>[6x]M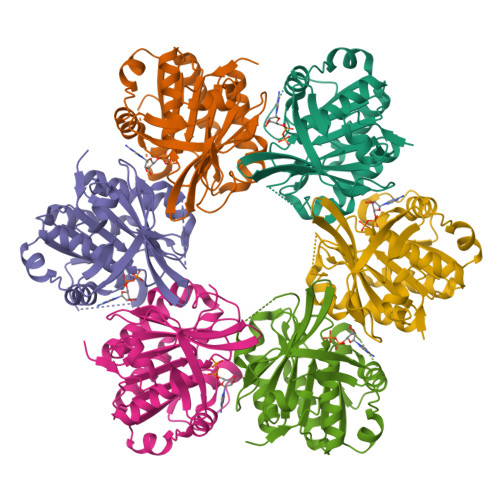TRRVKTGIPGVDEILHGGIPERNVVLLSGGPGTGKTIFSQQFLWNGLKMGEPGIYVALEEHPVQVRQNMAQFGWDVKPYEEKGMFAMVDAFTAGIGKSKEYEKYIVHDLTDIREFIEVLRQAIRDINAKRVVVDSVTTLYINKPAMARSIILQLKRVLAGTGCTSIFVSQVSVGERGFGGPGVEHGVDGIIRLDLDEIDGELKRSLIVWKMRGTSHSMRRHPFDITDKGIIVYPDKVLKRGKVLEL> MDPLNRRQFLALAAAAAGVTAGCAGMGGGGSVKSGSGPIDFWSSHPGQSSAAERELIGRFQDRFPTLSVKLIDAGKDYDEVAQKFNAALIGTDVPDVVLLDDRWWFHFALSGVLTALDDLFGQVGVDTTDYVDSLLADYEFNGRHYAVPYARSTPLFYYNKAAWQQAGLPDRGPQSWSEFDEWGPELQRVVGAGRSAHGWANADLISWTFQGPNWAFGGAYSDKWTLTLTEPATIAAGNFYRNSIHGKGYAAVANDIANEFATGILASAVASTGSLAGITASARFDFGAAPLPTGPDAAPACPTGGAGLAIPAKLSEERKVNALKFIAFVTNPTNTAYFSQQTGYLPVRKSAVDDASERHYLADNPRARVALDQLPHT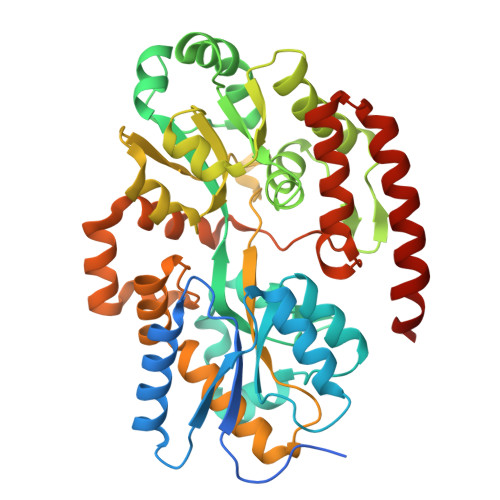RTQDYARVFLPGGDRIISAGLESIGLRGADVTKTFTNIQKRLQVILDRQIMRKLAGHG> TRECIYYNANWELERTNQSGLERCEGEQDKRLHCYASWRNSSGTIELVKKGCWLDDFNCYD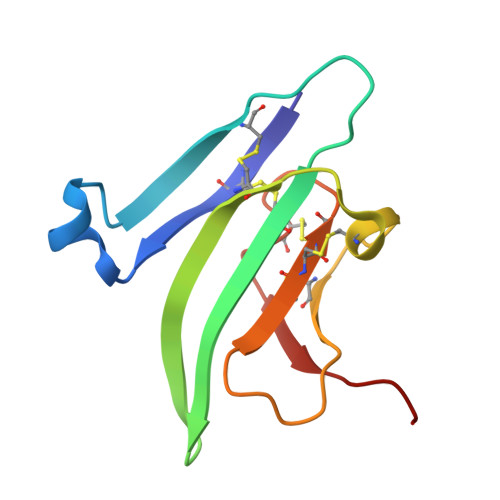RQECVATEENPQVYFCCCEGNFCNERFTHLPEPG~{N}-methyl-3-[[6-(2-methylpyrazol-3-yl)-1-oxidanylidene-isoquinolin-2-yl]methyl]benzamide 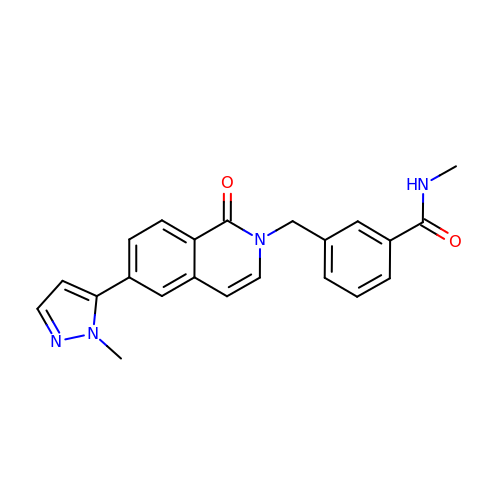| C22 H20 N4 O2 | MWHJTNPZZGOHMN-UHFFFAOYSA-N3-[(3-fluoro-4-methoxybenzyl)amino]-6-(trifluoromethyl)quinoxaline-2-carboxylic 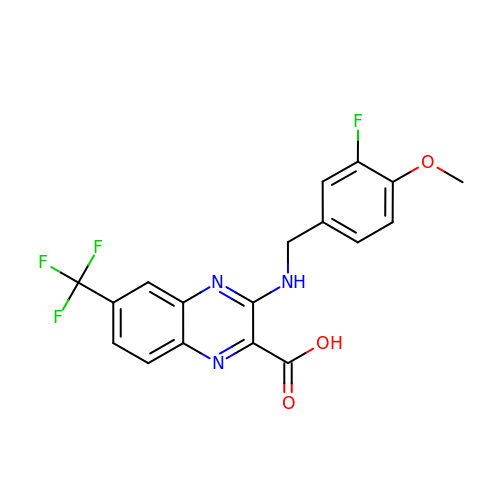acid | C18 H13 F4 N3 O3 | JKKOLPWDKQDVJE-UHFFFAOYSA-N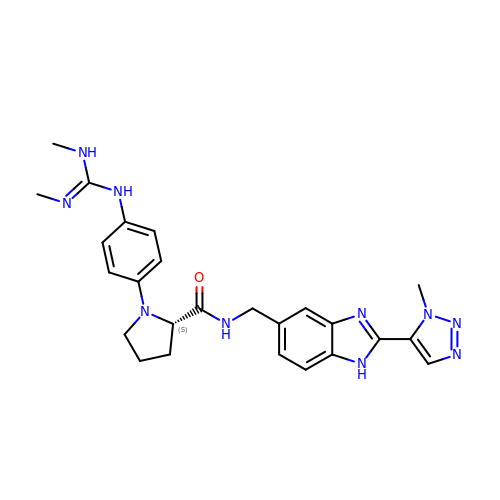(2~{S})-1-[4-[[(~{E})-~{N},~{N}'-dimethylcarbamimidoyl]amino]phenyl]-~{N}-[[2-(3-methyl-1,2,3-triazol-4-yl)-1~{H}-benzimidazol-5-yl]methyl]pyrrolidine-2-carboxamide | C25 H30 N10 O | MXOKQNYTQUSCFY-NRFANRHFSA-N>GSHMAKTYDYLFKLLLIGDSGVGKTCVLFRFSEDAFNSTFISTIGIDFKIRTIELDGKRIKLQIWDTAGLERFRTITTAYYRGAMGIMLVYDITNEKSFDNIRNWIRNIEEHASADVEKMILGNKCD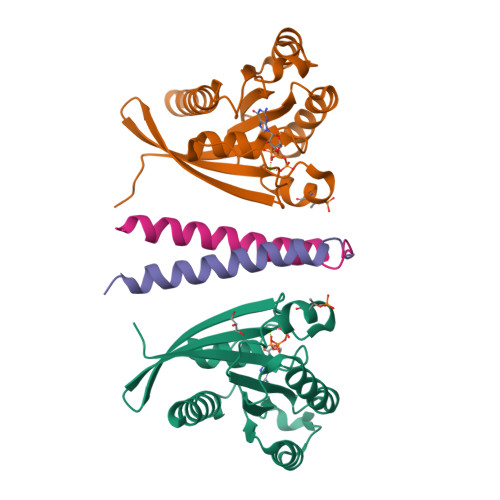VNDKRQVSKERGEKLALDYGIKFMETSAKANINVENAFFTLARDIKAKMDKKLEGNS[2x];>[2x]HHHHHHNRPRFTLQELRDVLQERNKLKSQLLVVQEELQCYKSG>[2x]GA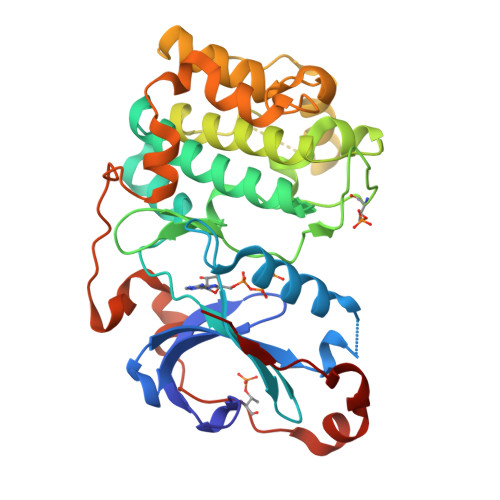MDPLGLQDFDLLRVIGRGSYAKVLLVRLKKTDRIYAMKVVKKELVNDDEDIDWVQTEKHVFEQASNHPFLVGLHSCFQTESRLFFVIEYVNGGDLMFHMQRQRKLPEEHARFYSAEISLALNYLHERGIIYRDLKLDNVLLDSEGHIKLTDYGMCKEGLRPGDTTSTFCGTPNYIAPEILRGEDYGFSVDWWALGVLMFEMMAGRSPFDIVGSSDNPDQNTEDYLFQVILEKQIRIPRSLSVKAASVLKSFLNKDPKERLGCHPQTGFADIQGHPFFRNVDWDMMEQKQVVPPFKPNISGEFGLDNFDSQFTNEPVQLTPDDDDIVRKIDQSEFEGFEYINPL> GSHMAAIESFDHIYLDLSKEPGKCRFAENGLGWKPVGGGETF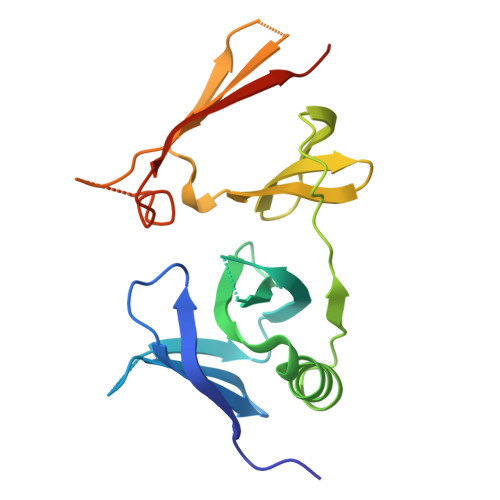TLDVSNIGGAQWSRAARGYEVKILQRTSGVIQLDGFQQEDYERLAKIFKNWYSTNLENKEHSLRGWNWGKAEFGKAELTFNVQNRPAFEIPYSEIANTNLAGRNEIAVEFAPGDHGKSSQNGQVKSKKASASRDQLVEIRFYIPGTTTRKEAE>GSAMGSDTVIDEKINIPVPLGTVFSLLYGDDTSYIKKIIENQNNFNVCDIPKFVNNAREITYTKKLNNSFGPKQTKCIVTETIEHMDLNSFFMVKQIVRSPDVPYGSSFSVHTRFFYSWGDHNTTNMKVVTNVVWTGKSMLK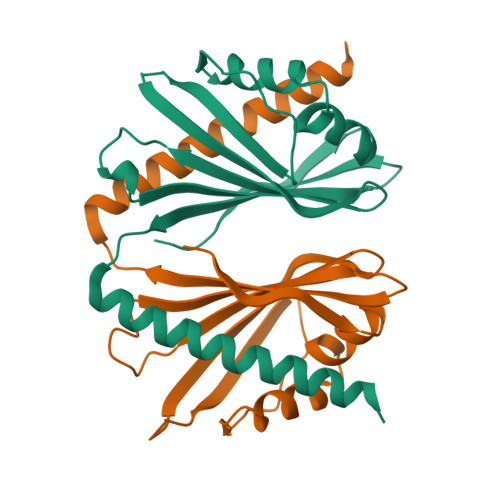GTIEKGSIDGQRSSTKQLVDDLKKIISN[2x]> MKNIFFICFCALFAFSGCADDDDDLLTGGNVDIDLLPDAKPNDVVDPQVFEAINLNYPGLEKVKEFYEAGEHYYAANALLEYYRTRTNVTNPNLSLINVTISEAEQAKADYALV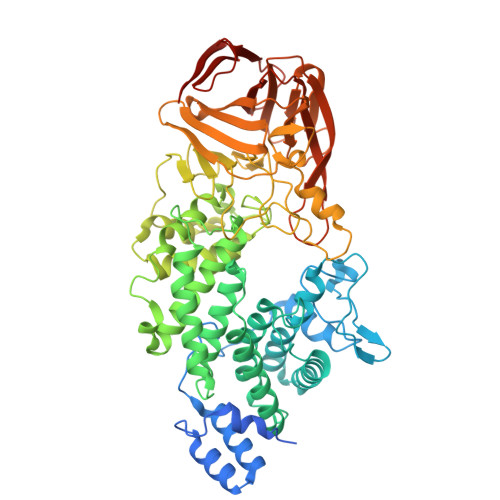DYRFHVNNFYEDKETLKPYSVKQDGGINWEYSPKDASDEYQKQLHRHQWFIPQAKAYRVSGDEKYIQSWIEVYKNWIENNPKPTTGPNTTSWWQLQVSTRIGDQVQLLEYFKNSVNFTPEWLSTFLVEFAEQADFLVDYPYESGGNILISQANALATAGTLMPEFKNAEKWMNTGYQILSEEVQNQIMSDGWHKEMSLHYHIGIVADFYEAMKLAEANQLSSKLPSDFTEPLRKAAEVVMYFTYPNYFIKGSDNVVPMFNDSWSRTRNVLKNTNFKQYVEMFPDSEELKYMQTAGNGGTAQGRTPNNDMKLFDQAGYYVLRNGWTPASTVMILSNNKSNDASNSLSAYSHNQPDNGTFELYHNGRNFFPDSGVCTYYTSGGDNDLRYWFRGIDKHNTLSIGKQNIKKAAGKLLKSEEGATELVVFENQGYDNLKHRRAVFYVNKKFFVLVDEGIGNAEGTINLSFNLCEGTASEVVMDTDKNGVHTAFSNNNNIIVRTFANKAVTCSPFTGRIAYLVDGAYNTRQSYTIDMNKSADETARYITVILPVNGSTDTSSISAKFIDSGYSENSASVEVSVNGETHTLSYTL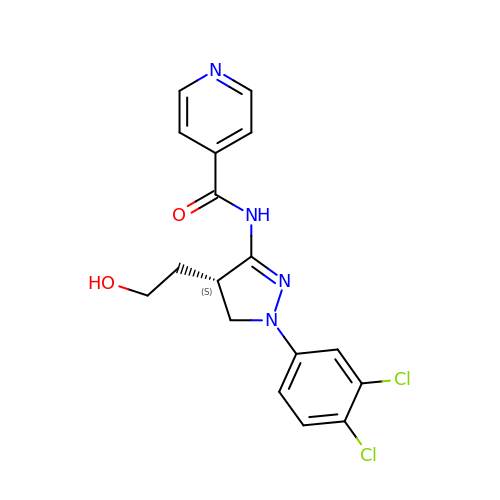~{N}-[(4~{S})-2-(3,4-dichlorophenyl)-4-(2-hydroxyethyl)-3,4-dihydropyrazol-5-yl]pyridine-4-carboxamide | C17 H16 Cl2 N4 O2 | XHACMMNMQIKLAQ-LBPRGKRZSA-N>EAGGVFKLIANDGKADRMIMANDLLNDRIKSIMCLRAKQGFSDPTPTLVDIERTHILLINSHYKPFAAMGYEYQKTRPNTGNPTYNSTIQFSIPQFGDFFSDMVVHVQLAATSASAGTVPALPAFIGADDQVLTSTSVVSATENTTSGVYTLYTQSYVNQQGTTQTVAAAATNFVRYCEYPGLRLFKRVKFEVNGNPLDEYTALAAIMYNKFHVPDFKLTGWKRLIGQEVPVEAASNLVNIASTTPWGSPIVALSDVNGTAVTGSPVNAAITARKLTQVVFGAQTPKATQEQLNMFVPLLFWFRDPRLAIASVSIPYGQRFITVDIEQQSNILFTAPGNLFLQTTVETLLTTGAGKGTATGVLLTQYNRYTTYT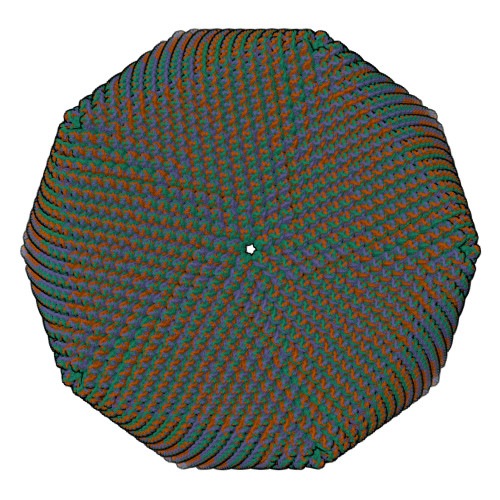PTLASGSSIDGTQAVQNIELYINNIFVTPEIHDIYIKRIGFTLIRVYREQVQREVNAADQVLQSQLKWPVEFIYLGLRPANNIAAGNTYQWRDWHHLTSVTNEPVYDVSQSYARVSIDDTVAPVGSTTFKQSASQVMQNQYIVPVETETLDTVRVKAHGIELYAQYRAQFYRDYIPWNYGSFNLVTPQDKGALFLNFCLYPGTYQPSGHVNISRAREFYIEYTSSFCDSSNPCDLISIAKCINFLLISDGSAVLRYSTKEFYLQCLILRCI[3x]>LEAKKEENLADWYSQVITKSEMIEYHDISGCYILRPWAYAIWEAIKDFFDAEIKKLGVENCYFPMFVSQSALEKEKTHVADFAPEVAWVTRSGKTELAEPIAIRPTSETVMYPAYAKWVQSHRDLPIKLNQWCNVVRWEFKHPQPFLRTREFLWQEGHSAFATMEEAAEEVLQILDLYAQVYEELLAIPVVKGRKTEKEKFAGGDYTTTIEAFISASGRAIQGGTSHHLGQNFSKMFEIVFEDPKIPGEKQFAYQNSWGLTTRTIGVMTMVHGDNMGLVLPPRVACVQVVIIPCGITNALSEEDKEALIAKCNDYRRRLLSVNIRVRADLRDNYSPGWKFNHWELKGVPIRLEVGPRDMKSCQFVAVRRDTGEKLTVAENEAETKLQAILEDIQVTLFTRASEDLKTHMVVANTMEDFQKILDSGKIVQIPFCGEIDCEDWIKKTTARDQDLEPGAPSMGAKSLCIPFKPLCELQPGAKCVCGKNPAKYYTLFGRSY[2x]

PARS1 is one of the aminoacyl‐tRNA synthetases (ARSs), which mediate the covalent ligation of amino acids to their cognate tRNAs for protein synthesis (Kim et al, 2011; Kwon et al, 2019). PARS1 catalyzes the covalent linkage of proline to tRNAPro. Unlike the other ARSs, PARS1 exists as a part of the bifunctional enzyme, glutamyl‐prolyl‐tRNA synthetase 1 (EPRS1), which comprises glutamyl‐tRNA synthetase 1 (EARS1), three repeats of WHEP domain, and PARS1 (Kwon et al, 2019). PARS1 is a homodimer formed by the PARS1 protomers A and B (Zhou et al, 2013).

DWN12088 and DWN11251 bound to PARS1 protomers asymmetrically (compounds with asymmetric binding, ABC), whereas HF, DWN11748, and DWN11761 bound symmetrically (compounds with symmetric binding, SBC). More specifically, protomers A and B of SBC‐bound PARS1 and protomer A of ABC‐bound PARS1 showed similar structures to each other, whereas protomer B of ABC‐bound PARS1 was different from the others in terms of the binding of both ATP and the compounds. The electron density map of ATP in protomer B of the DWN11251‐bound structure was also unclear compared with the others. Protomer B of the DWN11251‐bound structure also showed the decreased number of hydrogen bonds compared with protomer A. When comparing the number of hydrogen bonds of protomers A and B with each compound, relatively similar numbers of hydrogen bonds were counted in the complexes with SBC. In contrast, protomer A made over 10 more hydrogen bonds than protomer B in the complexes with ABC, implying the flexible or weakened binding of ATP in PARS1 protomer B. Another ABC, DWN11251, had a ketone group in the bridge, unlike DWN12088, and the halogen substituent of the bicyclic ring in HF was changed to a halogenated benzyl group, making the structure bulkier (Fig EV5C). In protomer A, halogen atoms in HF and DWN12088 showed an optimal distance to H1093 of 3.36–4.26 Å, and the distance between H1093 and the fluoride group in DWN11251 was 3.22 Å. On the other hand, since the distance was very close (2.2 Å) in DWN11251‐bound protomer B, the R‐loop was not stabilized due to the van der Waals repulsion or steric hindrance with halogen atom, possibly resulting in the unstable binding of DWN11251 to the R‐loop in protomer B. Overall, the flexibility of the A‐loop and R‐loop in the PARS1‐compound complex structures seemed to be responsible for the different binding modes between ABC and SBC. ABC showed relatively wide margins and gentle slopes while SBC showed narrow margins and steep slopes.>GSGFQIPATITERYKVGRTIGDGNFAVVKECVERSTAREYALKIIKKSKCRGKEHMIQNEVSILRRVKHPNIVLLIEEMDVPTELYLVMELVKGGDLFDAITSTNKYTERDASGMLYNLASAIKYLHSLNIVHRDIKPENLLVYEHQDGSKSLKLGDFGLATIVDGPLYTVCGTPTYVAPEIIAETGYGLKVDIWAAGVITYILLCGFPPFRGSGDDQEVLFDQILMGQVDFPSPYWDNVSDSAKELITMMLLVDVDQ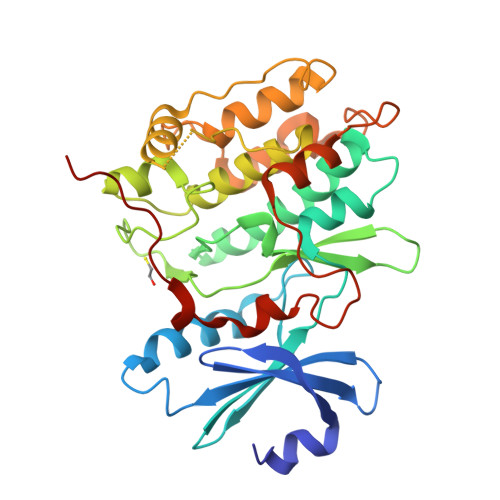RFSAVQVLEHPWVNDDGLPENEHQLSVAGKIKKHFNTGPKPNSTAAGVSVIATTALDKERQVFRRRRNQD[2x]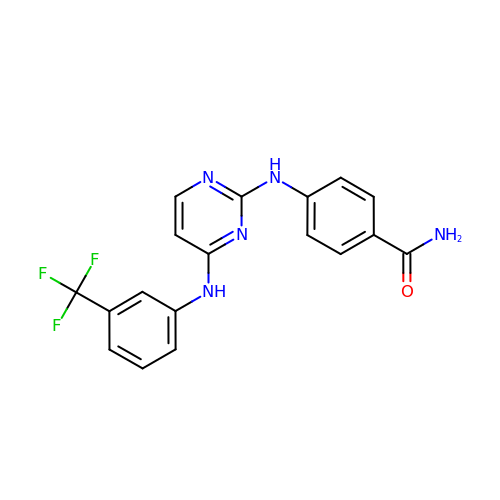4-[(4-{[3-(trifluoromethyl)phenyl]amino}pyrimidin-2-yl)amino]benzamide | C18 H14 F3 N5 O | WTPGNNPEEJSILJ-UHFFFAOYSA-N>[3x]NGHLQ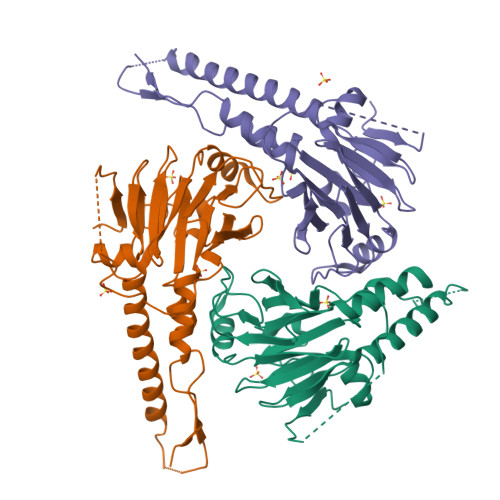HHPPMPPHPGHYWPVHNELAFQPPISNHPAPEYWCSIAYFEMDVQVGETFKVPSSCPIVTVDGYVDPSGGDRFCLGQLSNVHRTEAIERARLHIGKGVQLECKGEGDVWVRCLSDHAVFVQSYYLDREAGRAPGDAVHKIYPSAYIKVFDLRQCHRQMQQQAATAQAAAAAQAAAVAGNIPGPGSVGGIAPAISLSAAAGIGVDDLRRLCILRMSFVKGWGPDYPRQSIKETPCWIEIHLHRALQLLDEVLHTMPIADPQPLD>GAMTRIAINGFGRIGRLVFRAGIKDPNLEFVAINDLVTPDNLAYLLKYDSTHGRFQGTVEHTEKELIVDGKKILCVSERDPEKLPWKDLKVDYVIESTGLFTDRVGAEKHIKAGAKKVVISAPAKDKDIPTFVMGVNNEKYNPSNDHIVSNASCTTNCLAPIVKVVLDNWGIEEGLMTTIHATTATQPTVDGPSKKDFRGGRGAMQNIIPASTGAAKAVGLCIPEVNGKLTGMSFRVPTPDVSVVDLTVRTTKETSLKEISAKMKAASEGAMKGILGYTEDMVVSNDFVSSTLSSIFDMDACIELNSRFFKLVSWYDNEMGYSNRVLDLIRYMAKKG[8x]

In this work, we have solved the X-ray crystallographic structure of L. interrogans glyceraldehyde-3-phosphate dehydrogenase (GAPDH) to 2.37-Å resolution, a glycolytic enzyme that has been shown to exhibit moonlighting functions that potentiate infectivity and immune evasion in various pathogenic organisms. Besides carrying out moonlighting functions in the extracellular space, LiGAPDH is a glycolytic enzyme located in the cytoplasm. The quaternary structure of LiGAPDH consists in a homotetramer with O, P, Q, and R subunits related by a 222/D2 molecular symmetry, which gives rise to three non-equivalent interfaces related by three mutually perpendicular axes referred to as P, Q, and R. The monomers are composed of two domains: an N-terminal domain that contains the NAD+ binding pocket (residues 1-152), and a catalytic C-terminal domain spanning residues 153-335.

The crystal structure corresponds to the holoenzyme with an NAD+ molecule tightly bound into the active site. There are two independent tetramers in the asymmetric unit that are nearly identical, with an r.m.s.d. of 0.30 Å. The N-terminal domain adopts an α/β/α Rossmann fold characterized by the classic α/β nucleotide binding pocket, which typically contains a central 7-stranded β-sheet and a tightly bound NAD+ cofactor occupying the active site. In LiGAPDH there are 8 β-strands (β1 to β8) because the canonical seventh β-strand is split into two smaller β-strands (β7 and β8) by a small irregular segment of extended conformation. Another key structural feature of LiGAPDH is the S loop, an extended and irregular segment comprising residues Ala180-Ile207 that inserts itself between the NAD+-binding site and the adjacent subunit. At the bottom of the groove, the NAD+ cofactor occupies an elongated binding site between the central β-sheet of the N-terminal domain and helices H1-H5, where it makes contacts with the main-chain atoms of Asn32 (from β2), Glu76, and Arg77 (from the β5-310A loop). The catalytic Cys152 residue is located at the intersection between the N-terminal and C-terminal domains, where it interacts with the side chains of His179 and Arg234, the two other catalytic triad residues, responsible for lowering the pKa of the Cys152 thiol nucleophile. In contrast to other GAPDH structures, in LiGAPDH, well-ordered electron density was found for the residues responsible for binding the inorganic phosphate moieties of substrates and products, the so-called Ps and Pi binding sites. Inspection of the eight active sites in the crystal structure revealed that some of them had the Ps and Pi sites occupied by phosphate anions from the purification buffers or glycerol molecules from the cryoprotectant solution, which acted as substrates or substrate analogs. The crystallographic structure agrees with the solution SAXS data, suggesting that the crystal lattice has trapped the native conformation.> CDKSTDDTSKVTYFVTLEREGDEKIVLEKGQPFVEPGYYAEMNGEDITESVQIKGSVDVNTPGIYNLVYAAYNEDGFAKTFTRTVYVADNTASPLKSGIYTVAEGSKRTAPSVVAFSGYEIVIFQMEPGIFYISDFLGGWYDQRAGYGPDYAMVGKFELNDDNTITPLESYVA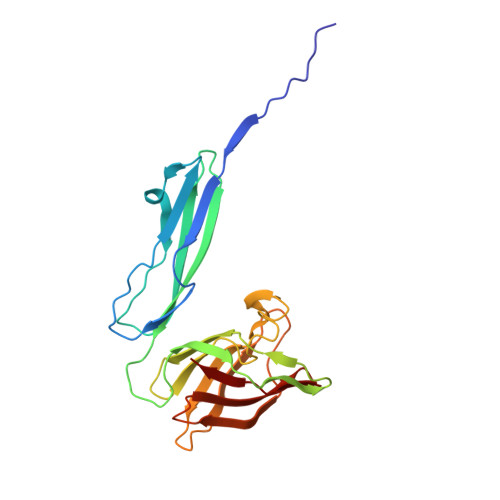GWGDSMDQMTNTLLDPATGTLKWTVAYAGQLSFDIIVKQ> MAEIYRKSAAETFTQLEATEKGLTTSEVTKRQEKYGFNELKNKKKDPLWKLFLETFKDPMVIVLVIAALVQLVLGEVVESLIIFLVLIVNSIISVVQTRKAESSLDALREMSAPVAKVIRDGSKQSIHARELVPGDVVILDAGDFVPADGRLFESGSLKIDEGMLTGESEAVEKYIDTIPDEVGLGDRVNMVF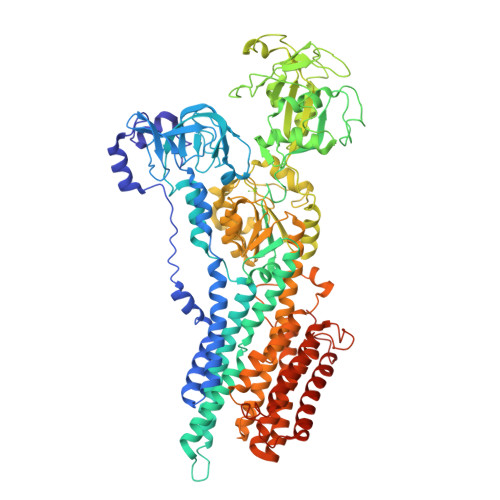SGSLVVYGRGMFVVTGTASETEIGKIAGLLETAEAKQTPLQRKLESFSKKLGLGILALCVLIFAVEAGRVLLGDNSADMATAILNAFMFAVAVAVAAIPEALSSIVTIVLAVGTNKMAKQHAIIRKLPAVETLGSTSVICTDKTGTLTQNKMTVVDYYLPDGTKENFPESPENWSEGERRLIHIAVLCNDSNINSEGKELGDPTEVALIAFSNKNNQDYNEIREKFIREGEIPFDSDRKLMSTLHTFNENKAMLTKGGPDVMFARCSYVFLDGEEKPMTEEILAKLKETNEEFSNQALRVLAYGYKRMPADTTELKLEDEQDIVLVGLTAMIDPPREAVYASIEESKKAGIRTVMITGDHKTTAQAIGRDIGLMDADDIALTGQELDAMPEEELDKKLEHIAVYARVSPENKIRIVKAWQKKGKITAMTGDGVNDAPALKQADIGVAMGSGTDVAKDSAAMILTDDNFVSIVDAVGVGRTVFDNIKKSIAYLFAGNLGAIIAILFALVLDWINPFTALQLLFINLVNDSLPAIALGMEKAEPDVMKRKPRDINEGIFAGGTMRAVISRGVLIGIAVIISQYIGMQISPEMSVAMAFTTLILARTLQTFAARSNVQTAFGAGFFSNKYVIGAVLLCFVLYGITVLPGAREIFSIPASFGLHEWSIAAGLALAAVVMMEIIKVVQNKFFKDYDIPTTENLYFQ> ASAKLPGDFGPPRGEPIHAV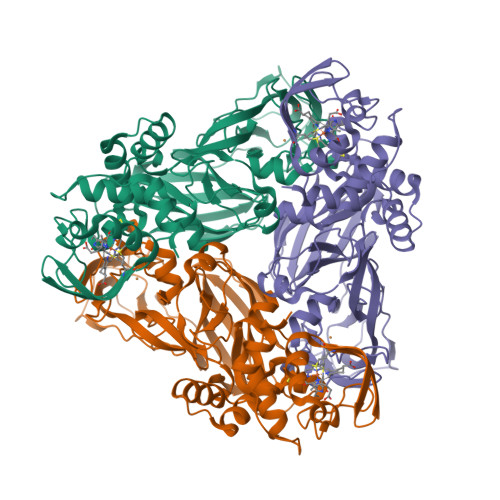LTSPPLVPPPVNRTYPAKVIVELEVVEKEMQISEGVSYTFWTFGGTVPGSFIRVRQGDTVEFHLKNHPSSKMPHNIDLHGVTGPGGGAASSFTAPGHESQFTFKALNEGIYVYHCATAPVGMHIANGMYGLILVEPPEGLPKVDHEYYVMQGDFYTAGKYREKGLQPFDMEKAIDERPSYVLFNGAEGALTGDKALHAKVGETVRIFVGNGGPNLVSSFHVIGAIFDQVRYEGGTNVQKNVQTTLIPAGGAAVVKFTARVPGSYVLVDHSIFRAFNKGAMAILKIDGAENKLVYSGKELDMVYLGDRAAPNMSAVTKATQASVSGTLTVQDQVQAGRALFAGTCSVCHQGNGAGLPGVFPPLAKSDFLAADPKRAMNIVLHGLNGKIKVNGQEYDSVMPPMTQLNDDEVANILTYVLNSWDNPGGRVSAEDVKKVRAQPAPAKAVAEH> HNMAGVGPGGYAAEFVPPPECPVFEPSWEEFTDPLSFIGRIRPLAEKTGIC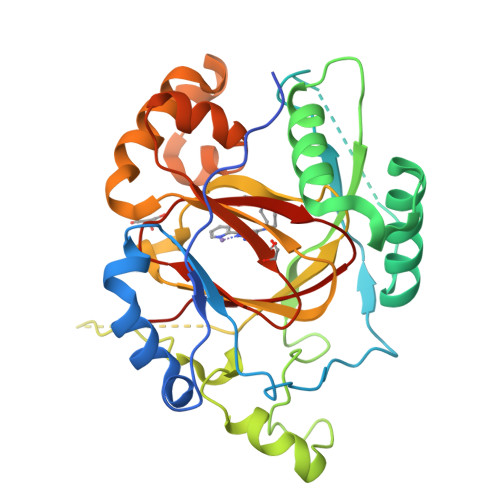KIRPPKDWQPPFACEVKSFRFTPRVQRLNELEAMTRVRPREAFGFEQAVREYTLQSFGEMADNFKSDYFNMPVHMVPTELVEKEFWRLVSSIEEDVIVEYGADISSKDFGSGFPVKDGRRKILPEEEEYALSGWNLNNMPVLEQSVLAHINVDISGMKVPWLYVGMCFSSFCWHIEDHWSYSINYLHWGEPKTWYGVPSHAAEQLEEVMRELAPELFESQPDLLHQLVTIMNPNVLMEHGVPVYRTNQCAGEFVVTFPRAYHSGFNQGYNFAEAVNFCT>SNAGNNDLKNVKAIAIVYRELSDGSQTVLLAKMKGLADEKGWMFVRGHVREDEEADPGVAAIRETQEETGFTGMVKKSGAPFTQPGSKDTQRVITIHPHIVQVQEASKSKDTEDTVKRQFLWVHPSEVRSKLQRAEMIQAWDQLHSFF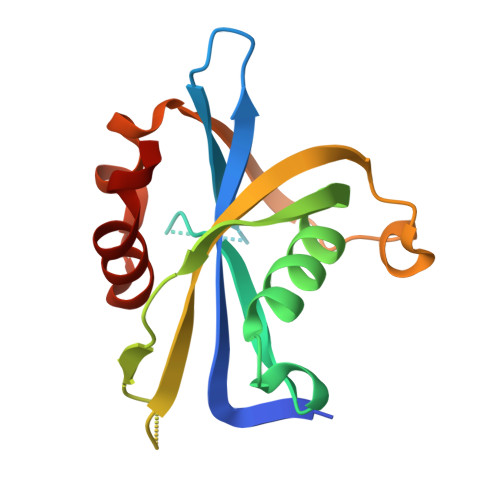[3x]>SQSRIFYLRNFNNWMKSVLIGEFLEKVRQKKKRDITVLDLGCGKGGDLLKWKKGRINKLVCTDIADVSVKQCQQRYEDMKNRRDSEYIFSAEFITADSSKELLIDKFRDPQMCFDICSCQFVCHYSFESYEQADMMLRNACERLSPGGYFIGTTPNSFELIRRLEASETESFGNEIYTVKFQKKGDYPLFGCKYDFNLEGVVDVPEFLVYFPLLNEMAKKYNMKLVYKKTFLEFYEEKIKNNENKMLLKRMGLGCLSKSEWEATSIYLVFAFEKQQ[2x]

RNA guanine-7 methyltransferase (RNMT) catalyses the transfer of a methyl group from S-adenosylmethionine (SAM) to the cap intermediate to form the cap m7G(5′)ppp(X) and the by-product S-adenosylhomocysteine (SAH). RNMT was identified based on homology to the yeast and viral homologues and in vitro activity. This basic cap structure (cap 0, m7G(5′)ppp(X)) protects RNA from degradation by nucleases during synthesis and recruits factors involved in RNA processing and translation initiation. RNMT has an activating co-factor RNMT-activating miniprotein (RAM) clamped at the interface of the catalytic domain and the modular lobe 416–456. Consequently, RNMT is a target of interest in cancers and immune disorders.

HsRNMT–Sinefungin–GMP-PnP, HsRNMT–SAH–DDD1060606 and HsRNMT–SAH–DDD1870799 co-complexes were solved, respectively, at 2.5, 2.0 and 2.4 Å in space group P21. The two inhibitors (DDD1060606 and DDD1870799) identified in the screening campaign were successfully co-crystallised with HsRNMT in the presence of SAH. DDD1870799 is also observed in the cap pocket of RNMT. In the presented structure, the pyrazolo-pyridine interacts with Y289 via two aromatic H-bonds, while the fluoro-benzene is buried in a hydrophobic pocket made by the residues including the main chain R173, as well as the side chains N176 and Y467. In comparison, the MIFs calculated for DDD1870799 suggest that the fluoro-phenyl moiety is responsible for the ligand binding via the interaction with a small pocket (S3) of high hydrophobicity. This interaction, by displacement of disorganised water molecules, is likely to be responsible for the significant gain in net enthalpic change ΔΔH measured for DDD1870799. However, a significant gain in net enthalpic change ΔΔH of −1.9 kcal/mol was measured for DDD1870799 in comparison with DDD1060606, suggesting that the interaction of DDD1870799 with HsRNMT-RAM is more enthalpy driven and might result in more selective leads with fewer absorption, distribution, metabolism, excretion and toxicity issues than DDD1060606. We report the structure of two small molecule inhibitors of RNMT as result of a diversity-driven hit discovery campaign. These molecules behave biochemically as uncompetitive inhibitors with respect to both cap and SAM despite the structural biology data leading to an expectation of competitive inhibition with cap. The biophysical data resolve this puzzle by demonstrating that the compounds require the presence of the enzymatic product, SAH, in RNMT to bind efficiently.> GGSTGGVPIQKVQDDTKTLIKTIVTRINDISHTQSVSAKQRVTGLDFIPGLHPILSLS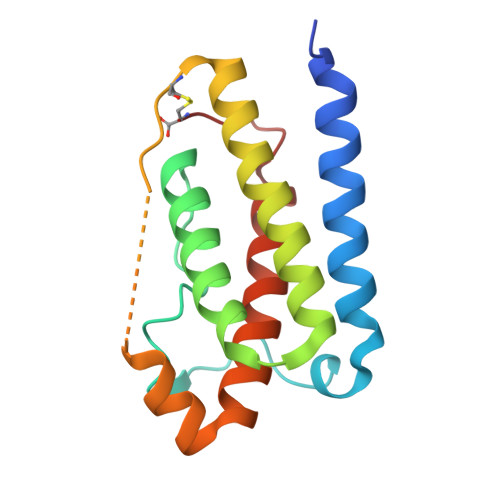KMDQTLAVYQQVLTSLPSQNVLQIANDLENLRDLLHLLAFSKSCSLPQTSGLQKPESLDGVLEASLYSTEVVALSRLQGSLQDILQQLDVSPEC> MDEAVQFSNASYEAAILENLALGT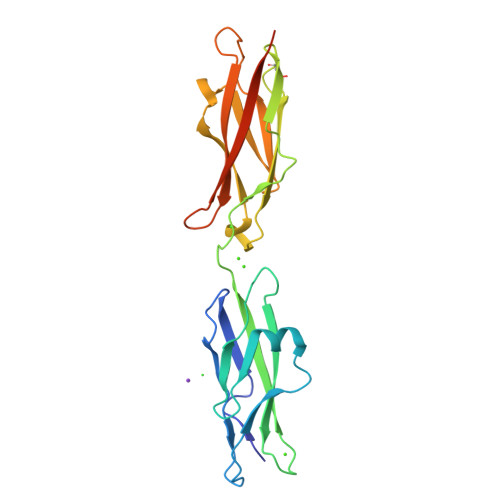EIVRVQAYSIDNLNQITYRFNAYTSTQAKALFKIDAITGVITVQGLVDREKGDFYTLTVVADDGGPKVDSTVKVYITVLDENDNSPRFDFTSDSAVSIPEDCPVGQRVATVKAWDPDAGSNGQVVFSLASGNIAGAFEIVTTNDSIGEVFVARPLDREELDHYILQVVASDRGTPPRKKDHILQVTILDINDNLEHHHHHH The TGF-β ligands are dimers and initiate signal transduction by forming a signalling complex with two copies of a type I receptor and two copies of a type II receptor; all are single-pass transmembrane proteins containing a small extracellular ligand-binding domain (ECD) and an intracellular kinase domain (ICD). Upon signalling complex formation, the constitutively active type II receptor phosphorylates and activates the type I receptor; subsequently the type I receptor phosphorylates Smad1/5 or Smad2/3 to regulate transcriptional responses. For example, ActRIIA/B bind to and mediate the signalling from both activin ligands and some BMP ligands, whereas BMPRII is the low-affinity type II receptor for over 15 BMP ligands. Of note, BMPRII is particularly highly expressed in lung vascular endothelial cells, where it mediates the signalling from circulating BMP9 and BMP10.

Here we also solved the crystal structures of BMP10 in a non-covalent complex with its prodomain (Pro:BMP10), which provided a BMP10 conformation in yet another protein interaction context. Two crystal forms were solved to 2.9 Å (crystal form 1, which contains Pro:BMP10 with mutations in the prodomain unstructured regions to promote crystal contacts), and to 3.5 Å (crystal form 2, which contains wild type (WT) Pro:BMP10), respectively. The two structures overlay well in the BMP10 chains and in the prodomain regions that interact with BMP10. The prodomain regions that are not engaged in protein-protein interactions and the α5 helix are truncated or disordered, i.e., not visible in the crystal structures. Importantly, the interface between the prodomain and BMP10 is identical in both structures and comprised of interactions from the extended β-sheet and the α2 helix, conserved with previously reported Pro:BMP9 structures. The four BMP10 monomers in the two Pro:BMP10 structures provided the conformation of BMP10 in the prodomain-bound form for further analysis. In the presence of the prodomain, the fingertip 3/4 is found in the bent conformation for both BMP9 and BMP10. Prodomain-binding fixes BMP9 and BMP10 in the bent conformation, presumably a more restrained conformation at least for BMP9 because the three free BMP9 structures, reported by different groups and using proteins purified by different methods, are all in the extended conformation.

>[2x]NAKGNYCKRTPLYIDFKEIGWDSWIIAPPGYEAYECRGVCNYPLAEHLTPTKHAIIQALVHLKNSQKASKACCVPTKLEPISILYLDKGVVTYKFKYEGMAVSECGCR;>SPIMNLEQSPLEEDMSLFGDVFSEQDGVDFNTLLQSMKDEFLKTLNLSDIPTQDSAKVDPPEYMLELYNKFATDRTSMPSANIIRSFKNEDLFSQPVSFNGLRKYPLLFNVSIPHHEEVIMAELRLYTLVQRDRMIYDGVDRKITIFEVLESKGDNEGERNMLVLVSGEIYGTNSEWETFDVTDAIRRWQKSGSSTHQLEVHIESKHDEAEDASSGRLEIDTSAQNKHNPLLIVFSDDQSSDKERKEELNEMISHEQLPELDNLGLDSFSSGPGEEALLQMRSNIIYDSTARIRR[2x]Using a phylogenomics-based approach and complementary structural techniques, we identify a family of dimeric hemoproteins comprising a domain of unknown function DUF2470. The heme iron is axially coordinated by two zinc-bound histidine residues, forming a distinct two-fold symmetric zinc-histidine-iron-histidine-zinc site. Together with structure-guided in vitro and in vivo experiments, we further demonstrate the existence of a functional link between heme binding by Dri1 (Domain related to iron 1, formerly ssr1698) and post-translational regulation of succinate dehydrogenase in the cyanobacterium Synechocystis, suggesting an iron-dependent regulatory link between photosynthesis and respiration. Given the ubiquity of proteins containing homologous domains and connections to heme metabolism across eukaryotes and prokaryotes, we propose that DRI (Domain Related to Iron; formerly DUF2470) functions at the molecular level as a heme-dependent regulatory domain. We heterologously expressed and purified the recombinant protein encoded by the Synechocystis gene dri1 (formerly known as ssr1698) and tested the heme-binding ability of this small, soluble protein (96 amino acids, 10 kDa).

His79Ala and His79Ala-Arg90Ala surprisingly bound heme. By comparison, the structure of His79Ala-Arg90Ala with heme has a similar dimer fold and interface as WT Dri1. Despite high R factors (Rwork/Rfree = 0.311/0.326) due to translational non-crystallographic symmetry, similar structural conformations were also obtained by SAXS-driven MD simulations (10−11). A slight rotation of ~30° of the plane of the heme is observed owing to the loss of His79. The remaining His side chains are equidistant from the heme iron (~4 Å N – Fe distances), likely contributing a weak interaction with the heme iron. Curiously, the absence of Arg90 permits the heme cofactor to rotate 180° such that the propionate groups interact with Arg12 at the N-termini. The slight planar rotation of heme with respect to the monomers observed in MD simulations can explain the relatively similar heme-binding ability of His79Ala-Arg90Ala to that of the WT protein. Hence, the function of His79 can be compensated for by the other His residues; loss of the His79 axial ligands allows His16 and His21 to interact with the heme iron, therefore highlighting the variability in heme binding when His79 is absent. SEC-SAXS studies indicate little to no changes in the dimer structure. CW-EPR spectra of His79Ala-Arg90Ala show that the heme iron remains in the high-spin (g = 6; S = 5/2) state regardless of zinc addition and is not bis-axially coordinated by amino acid side chains.

>[8x]MADPLTPAISDRICKHMNEDHASAIALYAQVFGQQTDVTMAQMQAIDPTGMDLVVESEGGSKTIRIEFEQPLKDSEDAAQVLIAMAKQAASVGKNSAENLYFQ N-[2-(2,5-Dioxopyrrolidin-1-yl)ethyl]-3-methylbenzamide | C14 H16 N2 O3 | 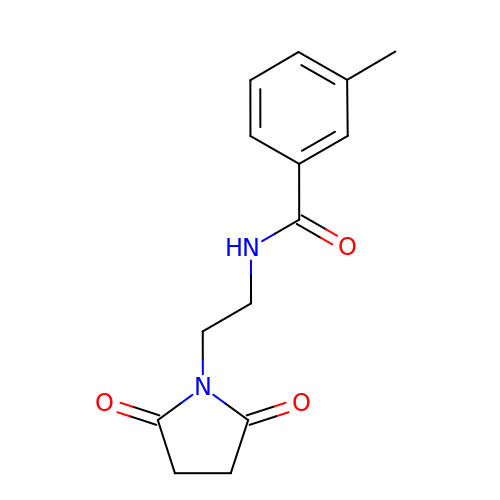YVZULSNTKFDGEM-UHFFFAOYSA-N>[2x]MNYARFITAASAARNPSPIRTMTDILSRGPKSMISLAGGLPNPNMFPFKTAVITVENGKTIQFGEEMMKRALQYSPSAGIPELLSWLKQLQIKLHNPPTIHYPPSQGQMDL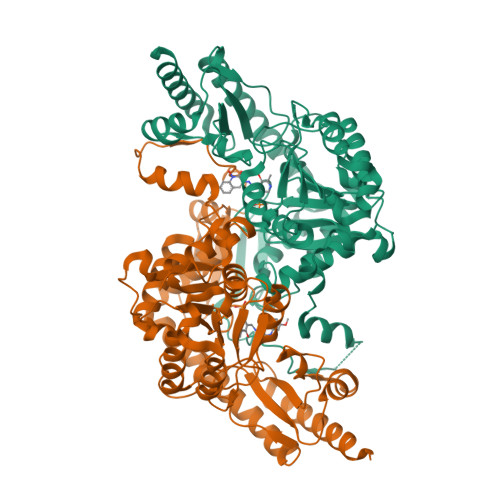CVTSGSQQGLCKVFEMIINPGDNVLLDEPAYSGTLQSLHPLGCNIINVASDESGIVPDSLRDILSRWKPEDAKNPQKNTPKFLYTVPNGNNPTGNSLTSERKKEIYELARKYDFLIIEDDPYYFLQFNSGRVPTFLSMDVDGRVIRADSFSKIISSGLRIGFLTGPKPLIERVILHIQVSTLHPSTFNQLMISQLLHEWGEEGFMAHVDRVIDFYSNQKDAILAAADKWLTGLAEWHVPAAGMFLWIKVKGINDVKELIEEKAVKMGVLMLPGNAFYVDSSAPSPYLRASFSSASPEQMDVAFQVLAQLIKESLLVPRGSLEHHHHHH> EEDLNWWEQENLRIAMKGERRWETLAHNGVLFPPEYEPHGIPIFYDGREFKMTPEEEEVATMFAVMKEHDYYRMEVFRRNFFESWREILDKRQHPIRRLELCDFEPIYQWHLVQREKKLSRTKEEKKAIKEKQDAEAEPYRYCVWDGRREQVANFRVEPPGLFRGRGKHPLMGKLKVRVQPEDITINIGETAEVPVPPAGHKWAAVQHDHTVTWLAMWRDSVAGNMKYVMLAPSSSVKGQSDMVKFEKARKLKDKVDDIRASYMEDFKSNDLHVAQRAVAMYFIDRLALRVGNEKGEDEADTVGCCSLRVEHIQLMPDNIVRFDFLGKDSIRYQNDVAVLPEVYALLQRFTRRKSPGMDIFDQLNPTQLNDHLKSFMDGLSAKVFRTYNASITLDRWFKEKPVDPKWSTADKLAYFNKANTEVAILCN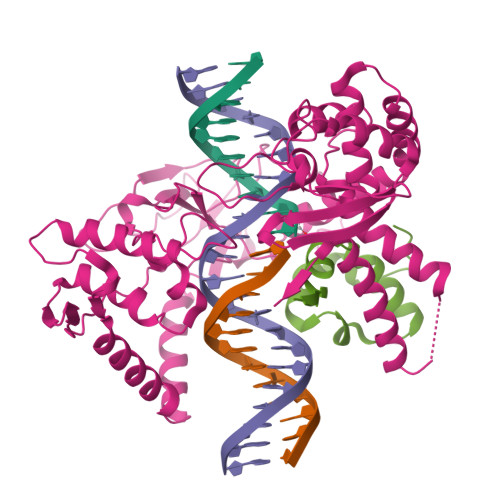HQKS;> ENIIRIKDDNKAVSLGTSKINYIDPRIICSWAKAQDVPINKIFSATIQKKFPWAMNAENFDF>[4x]MNMLVINGTPRKHGRTRIAASYIAALYH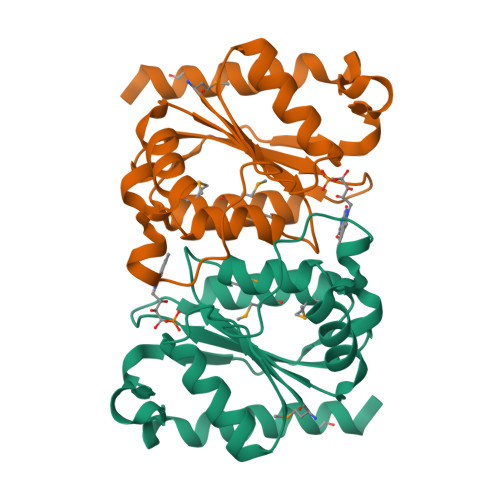TDLIDLSEFVLPVFNGEAEQSELLKVQELKQRVTKADAIVLLSPEYHSGMSGALKNALDFLSSEQFKYKPVALLAVAGGGKGGINALNNMRTVMRGVYANVIPKQLVLDPVHIDVENATVAENIKESIKELVEELSMFAKAGNPGVLEHHHHHH2-ethyl-2-methanoyl-~{N}-[3-[[4-(naphthalen-1-ylmethyl)piperazin-1-yl]methyl]phenyl]butanamide | C29 H35 N3 O2 | 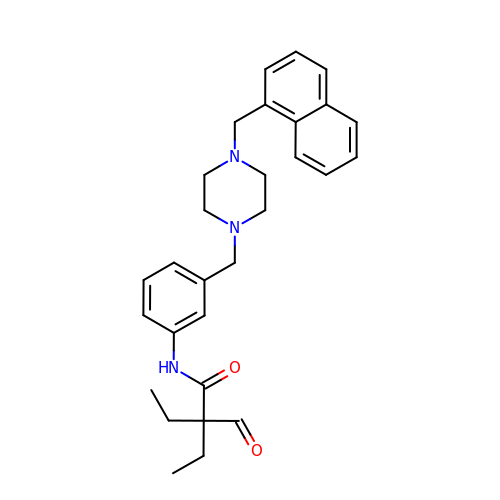AGJXNYANCJMTSI-UHFFFAOYSA-N>GAFTAQPQWPGASRRNNTGQEAVTDIRFLQSRAEHERAFTVFWRAMVGLPALGAVAADELLELGRYLGAFVQGELIGGADSYTSWLTVPGGSRVPHAAVTHIGVLPTHTRRGILTALVTRQLTDIAGRGEIVASLRASEAVIYRRFGYGIATSSATYRIQRRRAAPLRPIDTGAIALLDAAASPEGLAAIYERAAWTGSVARPPQWWRLHELFDAADPVKPYVVTHPDGYVRYRPQDTAEWFSSSARTISVDDLVAHSDEAYRALVG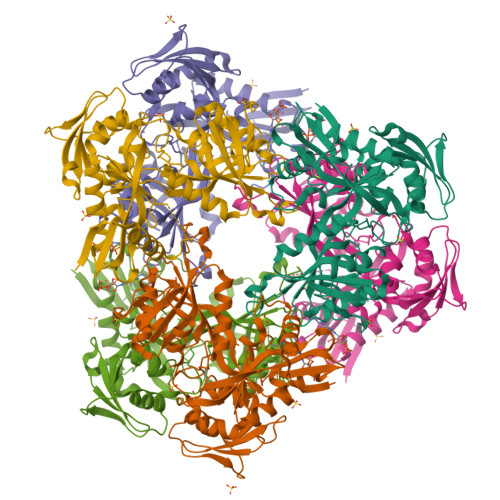HLLDLDLVDVIELGPRPIDDPLPHLVTDPRAVAVAGIRDETWLRLVDVEAALAARTYTDGAPVVIEVQDTLLPHNAARFSVSSDKVRRTQHTPDISVDVAALGSVYLGGNTWTRLERAGLVSAQSPGAIRAADALFSTGTQPFAGTNF[6x]2-[[3-(2-phenylethoxy)phenyl]amino]benzamide | C21 H20 N2 O2 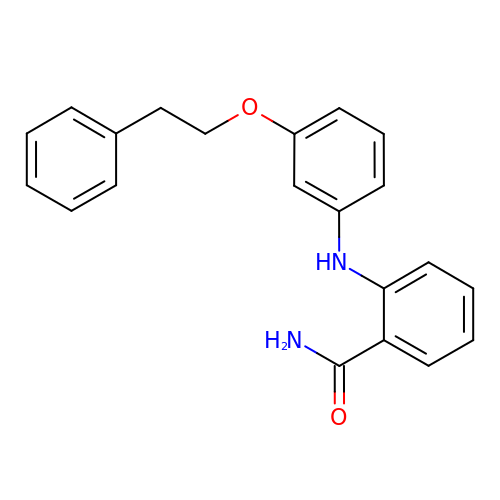| VVRUXFPJOVUDCV-UHFFFAOYSA-N> APVRSLNCGLRDSQQKSLVMSGPYELKALHLQGQDMEQQVVFSMSFVQGEESNDKIPVALGLKEKNLYLSCVLKDDKPTLQLESVDPKNYPKKKMEKRFVFNKIEINNKLEFESAQFPNWYISTSQAENMPVFL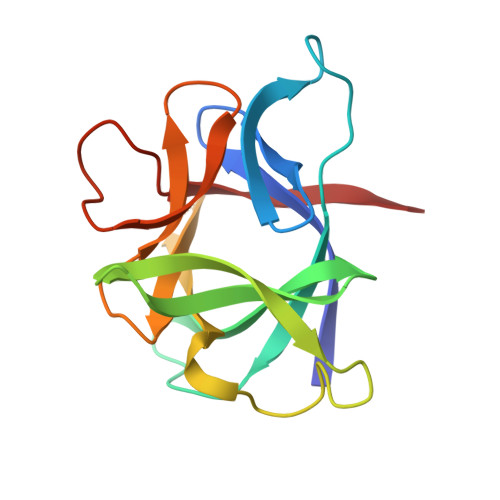GGTKGGQDITDFTMQFVSS> MS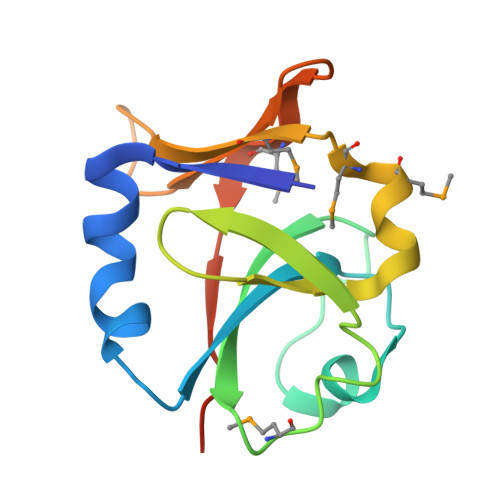LKITVTDDAAKKLQRYTDDSNAVLLLDFDDGVGALSKVGVCSLNSDFRILVVSKDMDYKKDYNEVIDSNIGKFYYKGYSKMYMDDNMKISLNTNNSLLRLTGDNSGELMPALSIQDFREGHHHHHH> MASQPNSSAKKKEEKGKNIQVVVRCRPFNLAERKASAHSIVECDPVRKEVSVRTGGLADKSSRKTYTFDMVFGASTKQIDV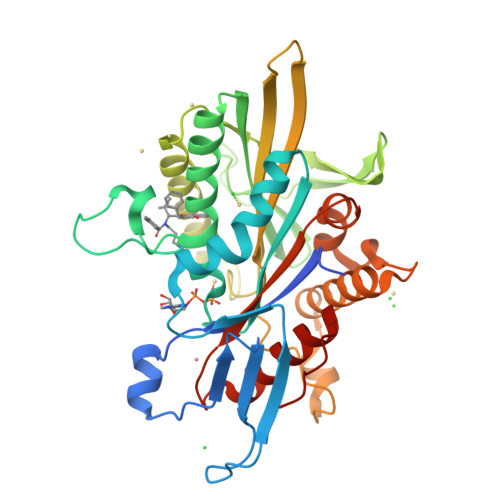YRSVVCPILDEVIMGYNCTIFAYGQTGTGKTFTMEGERSPNEEYTWEEDPLDGIIPRTLHQIFEKLTDNGTEFSVKVSLLEIYNEELFDLLNPSSDVSERLQMFDDPRNKRGVIIKGLEEITVHNKDEVYQILEKGAAKRTTAATLMNAYSSRSHSVFSVTIHMKETTIDGEELVKIGKLNLVDLAGSENIGRSGAVDKRAREAGNINQSLLTLGRVITALVERTPHVPYRESKLTRILQDSLGGRTRTSIIATISPASLNLEETLSTLEYAHRAKNILNKPEVNQK> ETPFTWEESNAYYWQPYALPL;> DKCKEREEKIILVSSANEIDVRPCPLNPNEHKGTITWYKDDSKTPVSTEQASRIHQHKEKLWFVPAKVEDSG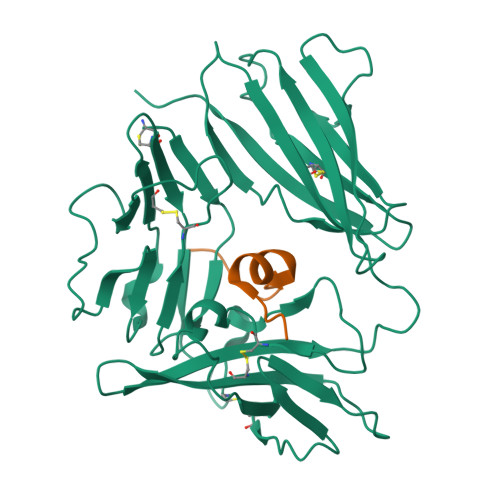HYYCVVRNSSYCLRIKISAKFVENEPNLCYNAQAIFKQKLPVAGDGGLVCPYMEFFKNENNELPKLQWYKDCKPLLLDNIHFSGVKDRLIVMNVAEKHRGNYTCHASYTYLGKQYPITRVIEFITLEENKPTRPVIVSPANETMEVDLGSQIQLICNVTGQLSDIAYWKWNGSVIDEDDPVLGEDYYSVENPANKRRSTLITVLNISEIESRFYKHPFTCFAKNTHGIDAAYIQLIYPVT>[2x]TYSTVSINTPPPYLTLACNEKLPTVLSIAGTDPSGGAGIEADVKTITAHRCYAMTC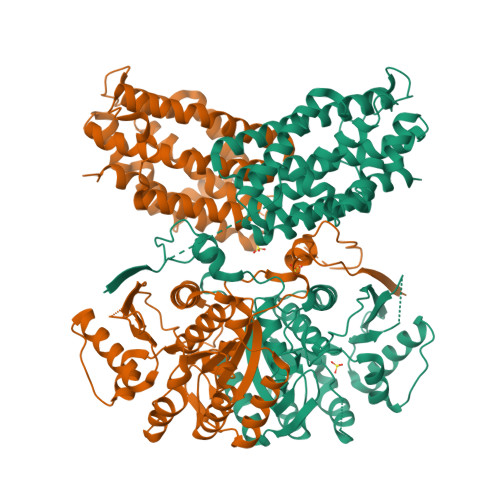ITALNAQTPVKVYSINNTPKEVVFQTLESNLKDMKCNVIKTGMLTAAAIEVLHEKLLQLGENRPKLVVDPVLVATSGSSLAGKDIVSLITEKVAPFADILTPNIPECYKLLGEERKVNGLQDIFQIAKDLAKITKCSNILVKGGHIPWNDEKEKYITDVLFLGAEQKFIIFKGNFVNTTHTHGTGCTLASAIASNLARGYSLPQSVYGGIEYVQNAVAIGCDVTKETVKDNGPINHVYAVEIPLEKMLSDECFTASDVIPKKPLKSAADKIPGGNFYEYLINHPKVKPHWDSYINHEFVKKVADGTLERKKFQFFIEQDYAYLVDYARVHCIAGSKAPCLEDMEKELVIVGGVRTEMGQHEKRLKEVFGVKDPDYFQKIKRGPALRAYSRYFNDVSRRGNWQELVASLTPCLMGYGEALTKMKGKVTAPEGSVYHEWCETYASSWYREAMDEGEKLLNHILETYPPEQLDTLVTIYAEVCELETNFWTAALEYE>[7x]MLDSLKSQFQPSFPRLASGHYVHFLMLRHSQSFPVFQTDGVLNTTRTQAGLLEKTDQLSRLVMFKRKQTTPERLAGRELLRNLGLTSADKSAKNLCEYNGEGSCKQCPDCILYGFAIGDSGSERSKVYSDSAFSLGAYEQSHRSFTFNAPFEGGTMSEAGVMRSAINELDHILPEVTFPTVESLRDATYEGFIYVLGNLLRTKRYGAQESRTGTMKNHLVGIVFADGEIFSNLHLTQALYDQMGGELNKPISELCETAATVAQDLLNKEPVRKSELIFGAHLDTLLQEVNDIYQNDAELTKLLGSLYQQTQDYATEFGALSGGKKKAKS;> MTKIYRCKLTLHDNVFFASREMGILYETEKYFHNWALSYAFFKGTIIPHPYGLVGQNAQTPAYLDRDREQNLLHLNDSGIYVFPAQPIHWSYQINTFKAAQSAYYGRSVQFGGKGATKNYPINYGRAKELAVGSEFLTYIVSQKELDLPVWIRLGKWSSKIRVEVEAIAPDQIKTASGVYVCNHPLNPLDCPANQQILLYNRVVMPPSSLFSQSQLQGDYWQIDRNTFLPQGFHYGATTAIAQDSPQLSLLDTN;> MTTLLQTLLIRTLSEQKDYILLEYFQTILPALEEHFGNTSGLGGSFISHQKHFGTQGYDTEKAKKMAQGFAKKGDQTLAAHILNALLTTWNVMQELEFPLNDIERRLLCLGITLHDYDKHCHAQDMAAPEPDNIQEIINICLELGKRLNFDEFWADWRDYIAEISYLAQNTHGKQHTNLISSNWSNAGYPFTIKERKLDHPLRHLLTFGDVAVHLSSPHDLVSSTMGDRLRDLLNRLGIEKRFVYHHLRDTTGILSNAIHNVILRTVQKLDWKPLLFFAQGVIYFAPQDTEIPERNEIKQIVWQGISQELGKKMSAGDVGFKRDGKGLKVSPQTSELLAAADIVRILPQVISVKVN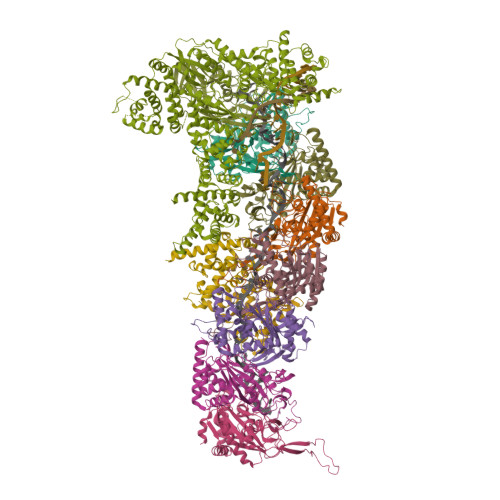NAKSPATPKRLEKLELGDAEREKLYEVADLRCDRLAELLGLVQKEIFLLPEPFIEWVLKDLELTSVIMPEETQVQSGGVNYGWYRVAAHYVANHATWDLEEFQEFLQGFGDRLATWAEEEGYFAEHQSPTRQIFEDYLDRYLEIQGWESDHQAFIQELENYVNAKTKKSKQPICSLSSGEFPSEDQMDSVVLFKPQQYSNKNPLGGGQIKRGISKIWSLEMLLRQAFWSVPSGKFEDQQPIFIYLYPAYVYAPQVVEAIRELVYGIASVNLWDVRKHWVNNKMDLTSLKSLPWLNEEVEAGTNAQLKYTKEDLPFLATVYTTTREKTDTDAWVKPAFLALLLPYLLGVKAIATRSMVPLYRSDQDFRESIHLDGVAGFWSLLGIPTDLRVEDITPALNKLLAIYTLHLAARSSPPKARWQDLPKTVQEVMTDVLNVFALAEQGLRREKRDRPYESEVTEYWQFAELFSQGNIVMTEKLKLTKRLVEEYRRFYQVELSKKPSTHAILLPLSKALEQILSVPDDWDEEELILQGSGQLQAALDRQEVYTRPIIKDKSVAYETRQLQELEAIQIFMTTCVRDLFGEMCKGDRAILQEQRNRIKSGAEFAYRLLALEAQQNQN;>MTEKLKLTKRLVEEYRRFYQVELSKKPSTHAILLPLSKALEQILSVPDDWDEEELILQGSGQLQAALDRQEVYTRPIIKDKSVAYETRQLQELEAIQIFMTTCVRDLFGEMCKGDRAILQEQRNRIKSGAEFAYRLLALEAQQNQN[2x]(1Z,3Z)-3-(2-phenylhydrazinylidene)-2,3-dihydro-1H-isoindol-1-imine 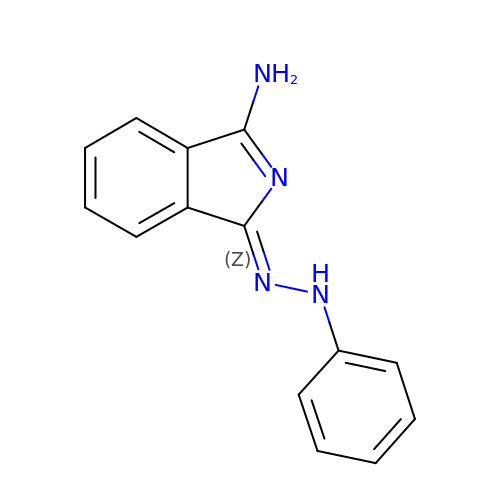| C14 H12 N4 | XBVFGEHZRVLBOS-UHFFFAOYSA-N> LVHVASVEKGRSYEDFQKVYNAIALKLREDDEYDNYIGYGPVLVRLAWHISGTWDKHDNTGGSYGGTYRFKKEFNDPSNAGLQNGFKFLEPIHKEFPWISSGDLFSLGGVTAVQEMQGPKIPWRCGRVDTPEDTTPDNGRLPDADKDAGYVRTFFQRLNMNDREVVALMGAHALGKTHLKNSGYEGPWGAANNVFTNEFYLNLLNEDWKLEKNDANNEQWDSKSGYMHLPTDYSLIQDPKYLSIVKEYANDQDKFFKDFSKAFEK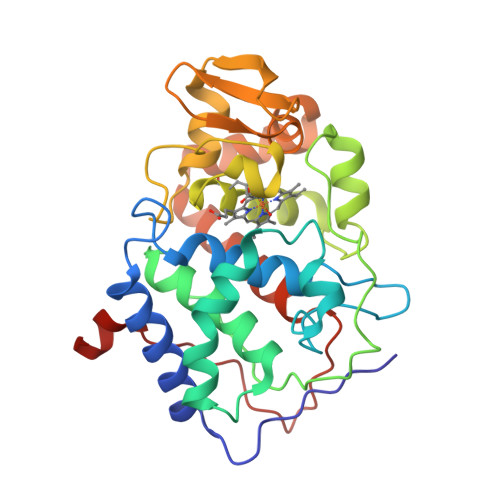LLENGITFPKDAPSPFIFKTLEEQGL>MSKSVFVGELTWKEYEARVAAGDCVLMLPVGALEQHGHHMCMNVDVLLPTAVCKRVAERIGALVMPGLQYGYKSQQKSGGGNHFPGTTSLDGATLTGTVQDIIRELARHGARRLVLMNGHYENSMFIVEGIDLALRELRYAGIQDFKVVVLSYWDFVKDPAVIQQLYPEGFLGF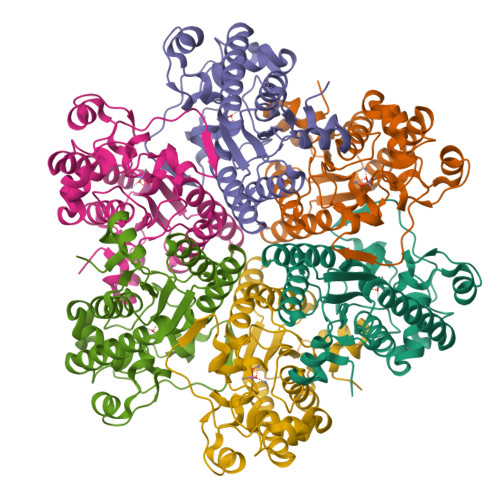DIEHGGVFETSLMLALYPDLVDLDRVVDHPPATFPPYDVFPVDPARTPAPGTLSSAKTASREKGELILEVCVQGIADAIREEFPPT[6x]(2R)-N-HYDROXY-2-[(3S)-3-METHYL-3-{4-[(2-METHYLQUINOLIN-4-YL)METHOXY]PHENYL}-2-OXOPYRROLIDIN-1-YL]PROPANAMIDE | C25 H27 N3 O4 | 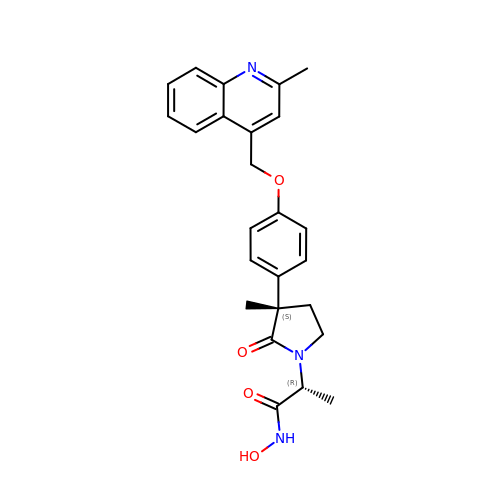YDMIPBHQKFOFQW-NSYGIPOTSA-N>MPSVYGARLTTFEDEEKESEYGYVRKVSGPVVIADGMNGAAMYELVRVGHDNLIGEIIRLEGDSATIQVYEETAGLMVNDPVLRTHKPLSVELGPGILGNIFDGIQRPLKTIAIRSGDVYIPRGVSVPALDKDTLWEFQPKKIGEGDLLTGGDLYATVFENSLMQHHVALPPDAMGKVTYVAPAGQYSLKDTVLELEFQGVKKSFTMLQAWPVRTPRPVSSKLAADTPLLTGQRVLDALFPSVLGGTCAIPGAFGCGKTVISQALSKYSNSDTVVYVGCGERGNEMAEVLMDFPQLTMTLPDGREESVMKRTTLVANTSNMPVAAREASIYTGITIAEYFRDMGYNVSMMADSTSRWAEALREISGRLAEMPADSGYPAYLAARLASFYERAGKVKCLGGPERTGSVTIVGAVSPPGGDFSDPVTSATLSIVQVFWGLDKKLAQRKHFPSVNWLISYSKYSTALESFYEQFDPDFINIRTKAREVLQREDDLNEIVQLVGKDALAEGDKITLETAKLLREDYLAQNAFTPYDKFCPFYKSVWMMRNIIHFYNLANQAVEKGAGMDGQKITYTLIKHRLGDLFYRLVSQKFEDPAEGEPALVAKFKKLHEDLTAGFRALEDETR[3x];>MGVAQNNVDMEEGTLEVAMEYRTVTGVAGPLVILDKVKGPKYYEIVNIRLGDGTMRRGQVLEVDGEKAVVQVFEGTSGIDNKFTTVQFTGEVLKTPVSLDMLGRIFNGSGKPIDNGPPILPEAYLDISGSSINPSERTYPEEMIQTGISTIDVMNSIARGQKIPLFSAAGLPHNEIAAQICRQAGLVKRLEKTDNLLEDGEEDNFAIVFAAMGVNMETAQFFKRDFEENGSMERVTLFLNLANDPTIERIITPRIALTTAEYLAYECGKHVLVILTDMSSYADALREVSAAREEVPGRRGYPGYMYTDLAQIYERAGRIEGRKGSITQIPILTMPNDDITHPTPDLTGYITEGQIYIDRQLQNRQIYPPINVLPSLSRLMKSAIGEGMTRRDHSDVSNQLYANYAIGKDVQAMKAVVGEEALSSEDLLYLEFLDKFERKFVAQGAYDSRNIFQSLDLAWTLLRIFPRELLHRIPGKTLDQYYSRDAAN[3x];>[3x]MNDADVSKQIQQMVRFIRQEAEEKANEISVSAEEEFNIEKLQLVEAEKKKIRQEYERKEKQVEIRKKIEYSMQLNASRIKVLQAQDDLVSNMMEAASKEVLNVSRDHNSYKKLLKGLIVQSLLRLKEPAVLLRCRKDDHHLVESVLESAKEEYAQKLQVHPPEIIVDHHIYLPPGPGHHNAHGPSCSGGVVVASRDGKIVCENTLDARLDVVFRKKLPEIRKQLVSQVAA;>MASNRGHGGIQQLLAAEQEAQHIVAAARNAKMARLRQAKEEAEREIAEHRAQVEREFQRKLAESSGDSGANVKRLEQETEVKIHHLNAGAEKIQYDVVQMLLKHVTTVKN[3x];> MAQNQRLTVVPTVTMLGVMKSRLVGATRGHALLKKKSDALTVQFRQILKNIVTTKESMGEVMKDSSFALIEAKYVAGENIKHIVLENVQNASIKVRSRQENIAGVKIPKFEYFTDGETKNDLTGLARGGQQVQQCRAAYVKAIELLVELASLQTSFLTLDEAIKTTNRRVNALENVVKPRLENTITYIKGELDELEREDFFRLKKIQGYKKREIERQLASSKQFVEEQFAEKVSLQKGISIKSAQNLLSAGEKDEDIIF;> MAGRAQIPTKSSALIAMIADEDTVTGFLLAGVGNVDLRRKTNYLIVDSKTTVKAIEDAFKEFTTKEDIAIVLISQYVANMIRFLVDSYNKPIPAILEIPSKDHPYDPAHDSVLSRVKNLFSAESVASGRR;> MASRYWVVSLPVQNSAASVWNRLQEQISKHSFDTPLYRFNIPNLRVGTLDSLLALSDDLVKSNSFVESVSHKIRRQIEELERVSGIESSSLSVDGVPVDTYLTRFVWDEAKYPTMSPLREIVDGIHTLVAKIEDDLKVRVAEYNNVRSQLNAINRKQSGSLAVRDLSNLVKPEDIITSEHLVTLLAVVPKYSQKDWLASYETLTSYVVPRSSKLLYEDNEYALYTVTLFGRVADNFRIAAREKGFQIRDFEYSSEAQESRNQELEKLVHDQESLRSSLLQWCYTSYGEVFSSWMHFCAVRVFAESILRYGLPPSFLACVLAPSVKGEKKVRSILEELCGNANSTFWKSEDDGGMMAGLGGDADSHPYVSFTINLV;> MDHAELTTEQVLKRDIPWETYMTTKLISGTGLQLLRRYDNRSESHRAQLLDDDGPSYVRVFVSILRDIYKEETVEYVLALIDEMLTANPKRARLFHDKSLASEDTYEPFLRLLWKGNWFIQEKSCKILASIVSARPKPQDRFFANGEASNSKSKSTTIDDVLKLLVEWLCAQLKKPSHPSRGVPVAINCLAALLKEPMVRSSFVQADGVKLLTPLISPASTQQSIQLLYETCLCVWLLSYYEPAVEYLATTRTLPRLIDVVKSSTKEKVVRVVVLILRNLLPKGNFAAQMIDLGLPQVVQSLKAQAWSDEDLLEGLNQLEEGLKDNIKRLSSFDKYKQEVLLGHLDWSPMHKDPLFWRDNITNFEENDFQILRVLLTILDTSSDPRALAVACFDLSQFIQYHPAGRVIVTDLKAKERVMKLMNHENTEVTKSALLCIQRLFLGAKYASFLQA;> MAELQSGGGGGCCPPMDLFRSEPMQLVQIIIPIESAHLTVSYLGELGLLQFKDLNSEKSPFQRTYAAQIKKCAEMARKLRFFKEQMLKAGILSSVKSTTRADNNTDDLEVKLGDLEAELVEINANGDKLQRAHSELVEYKLVLQKAGEFFSSALTSAAAQQREMESQQTGEMTIETPLLTDKEMSADPSKQIKLGFIAGLVPREKSMSFERMLFRATRGNVFLRQAVVDEPVVDPVSGEKMEKNVFVVFYSGERAKNKILKICDAFGANRYPFNEEFDKQAQAISEVSGRLSELKTTLDAGLLHRGNLLQTIGDQFEQWNLLVKREKSIYHTLNMLSLDVTKKCLVGEGWSPVFATKQIQDALERAAFDSNSQVGAIFQVLHTKESPPTYFRTNKFTSAFQEIVDAYGVAKYREANPGVFTIVTFPFLFAVMFGDWGHGICLLLGTLVLIVREKKLASQKLDDITDMTFGGRYVILMMALFSIYTGLIYNEFFSVPFEIFSHSAYACRDLSCSEATTVGLIKVRDTYPFGVDPVWHGSRSELPFLNSLKMKMSILLGVAQMNLGIILSYFNATFFRIGVNIWCQFIPQIIFLNSLFGYLSLLIILKWITGSQADLYHVMIYMFLSPTDELGDNQLFPGQKTAQLVLLLLAFVSVPWMLLPKPFILKMQHQDRHQGQSYEALQSTDESLQPDTNHDSHGHEEFEFSEVFVHQMIHTIEFVLGAVSNTASYLRLWALSLAHSELSSVFYEKVLLLAWGYNNILILIVGIIVFIFATVGVLLVMETLSAFLHALRLHWVEFQNKFYEGDGYKFSPFSFALLDDEDE;> MSGSVMLGESSSWSRALVKISPYTFSAIGIAVAIGVSVLGAAWGIYITGSSLIGAAIKAPRITSKNLISVIFCEAVAIYGVIVAIILQTKLESVPASQIYAPESLRAGYAIFASGIIVGFANLVCGLCVGIIGSSCA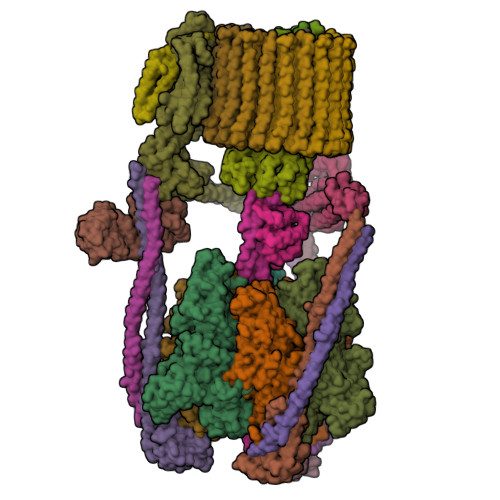LSDAQNSSLFVKILVIEIFGSALGLFGVIVGIIMSAQASWPAKPV;> MYGFEAMTFNIHGGYLEAIVRGYRAGLLTAADYNNLCQCETLDDIKMHLSATEYGPYLQNEPSPLHTTTIVEKCTLKLVDEYKHMLCQATEPLSTFLEYITYGHMIDNVVLIVTGTLHERDVQELLEKCHPLGMFDSIATLAVAQNMRELYRLVLVDTPLAPYFSECITSEDLDDMNIEIMRNTLYKAYLEDFYKFCQKLGGATAEIMSDLLAFEADRRAVNITINSIGTELTRDDRRKLYSNFGLLYPYGHEELAVCEDIDQVRGVMEKYPPYQSIFSKLSYGESQMLDKAFYEEEVKRLCLAFEQQFHYGVFFAYMRLREQEIRNLMWISECVAQNQKSRVHDSVVFIF;> MGFLVTTLVFLVIGIIASLCTRICCNRGPSTNLLHLTLVITATVSCWMMWAIVYLAQMKPLIVPILSEEE;>[9x]MSTFSGDETAPFFGFLGAAAALVFSCMGAAYGTAKSGVGVASMGVMRPELVMKSIVPVVMAGVLGIYGLIIAVIISTGINPKAKSYYLFDGYAHLSSGLACGLAGLSAGMAIGIVGDAGVRANAQQPKLFVGMILILIFAEALALYGLIVGIILSSRAGQSRAE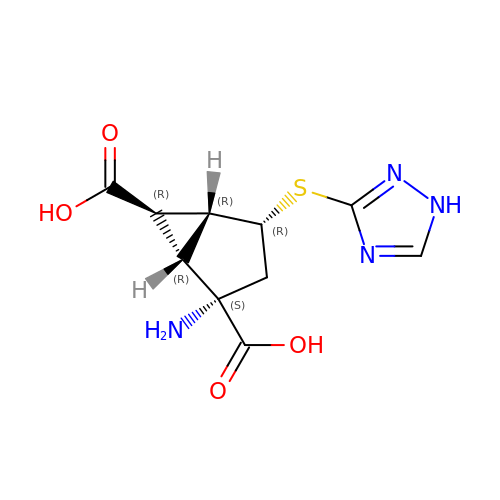(1R,2S,4R,5R,6R)-2-amino-4-(1H-1,2,4-triazol-3-ylsulfanyl)bicyclo[3.1.0]hexane-2,6-dicarboxylic acid | C10 H12 N4 O4 S | YSOWRGMLMZQSBX-AVUIYAGVSA-N>VQFRGGTTAQHATFTGAAREITVDTDKNTVVVHDGATAGGFPLARHDLVKTAFIKADKSAVAFTRTGNATASIKAGTIVEVNGKLVQFTADTAITMPALTAGTDYAIYVCDDGTVRADSNFSAPTGYTSTTARKVGGFHYAPGSNAAAQAGGNTTAQINEYSLWDIKFRPAALDPRGMTLVAGAFWADIYLLGVNHLTDGTSKYNVTIADGSASPKKSTKFGGDGSAAYSDGAWYNFAEVMTHHGKRLPNYNEFQALAFGTTEATSSGGTDVPTTGVNGTGATSAWNIFTSKWGVVQASGCLWTWGNEFGGVNGASEYTANTGGRGSVYAQPAAALFGGAWNGTSLSGSRAALWYSGPSFSFAFFGARGVCDHLIL[6x];>DWNNQSIIKAGERQHGIHIKQSDGAGVRTATGTTIKVSGRQAQGVLLENPAAELRFQNGSVTSSGQLFDEGVRRFLGTVTVKAGKLVADHATLANVSDTRDDDGIALYVAGEQAQASIADSTLQGAGGVRVERGANVTVQRSTIVDGGLHIGTLQPLQPEDLPPSRVVLGDTSVTAVPASGAPAAVSVFGANELTVDGGHITGGRAAGVAAMDGAIVHLQRATIRRGDAPAGGAVPGGAVPGGAVPGGFGPLLDGWYGVDVSDSTVDLAQSIVEAPQLGAAIRAGRGARVTVSGGSLSAPHGNVIETGGGARRFPPPASPLSITLQAGARAQGRALLYRVLPEPVKLTLAGGAQGQGDIVATELPPIPGA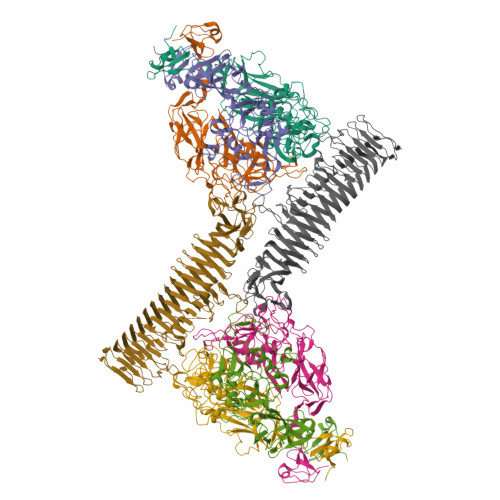SSGPLDVALASQARWTGATRAVDSLSIDNATWVMTDNSNVGALRLASDGSVDFQQPAEAGRFKVLMVDTLAGSGLFRMNVFADLGLSDKLVVMRDASGQHRLWVRNSGSEPASANTMLLVQTPRGSAATFTLANKDGKVDIGTYRYRLAANGNGQWSLVGAKAPP[2x]>[2x]VKTLCLRQNLIKCIENLEELQSLRELDLYDNQIKKIENLEALTELEILDISFNLLRNIEGVDKLTRLKKLFLVNNKISKIENLSNLHQLQMLELGSNRIRAIENIDTLTNLESLFLGKNKITKLQNLDALTNLTVLSMQSNRLTKIEGLQNLVNLRELYLSHNGIEVIEGLENNNKLTMLDIASNRIKKIENISHLTELQEFWM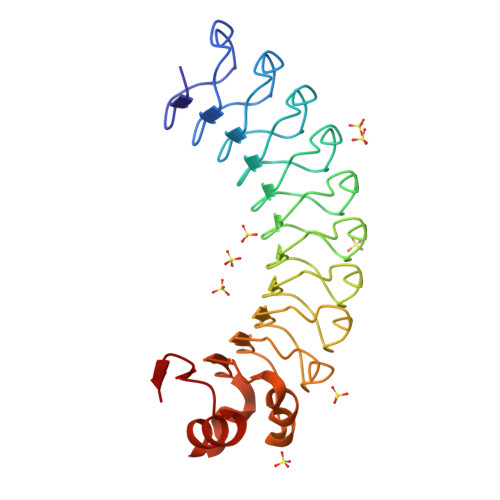NDNLLESWSDLDELKGARSLETVYLERNPLQKDPQYRRKVMLALPSVRQIDATFVRF>LSGAVTALILVIASVIIALVVV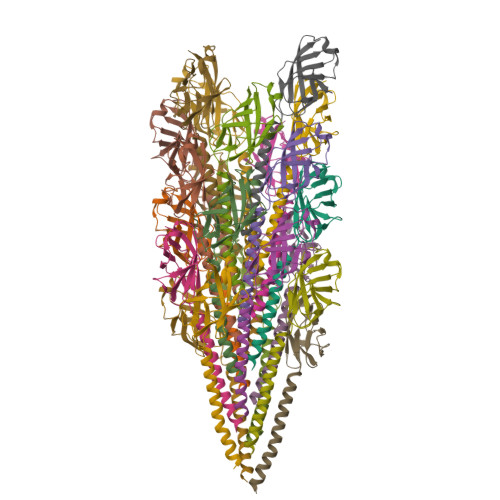GFAFGLFGAFTGQGTVTQVGTATLSASTGTLKVTLKNTGATTQVTGAIINGNAASVSGQVTISAGQSTYSISLGGISSSTLQSLVGSTISLTLQLSNGQTVTVSAIITS[21x]1-hydrazinophthalazine | C8 H8 N4 | 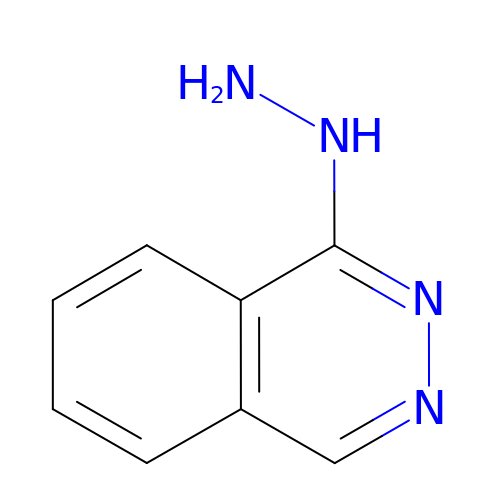RPTUSVTUFVMDQK-UHFFFAOYSA-N> DQQLVDQLSQLKLNVKMLDNRAGENGVDCAALGADWASCNRVLFTLSNDGQAIDGKDWVIYFHSPRQTLRVDNDQFKIAHLTGDLYKLEPTAKFSGFPAGKAVEIPVVAEYWQLFRNDFLPRWYATSGDAKPKMLANTDTENLDQFVAPFTGDQWKRTKDDKNILMTPASRFVSNADLQTLPAGALRGKIVPTPMQVKVHAQDADLRKGVALDLSTLVKPAADVVSQRFALLGVPVQTNGYPIKTDIQPGKFKGAMAVSGAYELKIGKKEAQVIGFDQAGVFYGLQSILSLVPSDGSGKIATLDASDAPRFPYRGIFLDVARNFHKKDAVLRLLDQMAAYKLNKFHFHLSDDEGWRIEIPGLPELTEVGGQRCHDLSETTCLLPQYGQGPDVYGGFFSRQDYIDIIKYAQARQIEVIPEIDMPAHARAAVVSMEARYKKLHAAGKEQEANEFRLVDQTDTSNTTSVQFFNRQSYLNPCLDSSQRFVDKVIG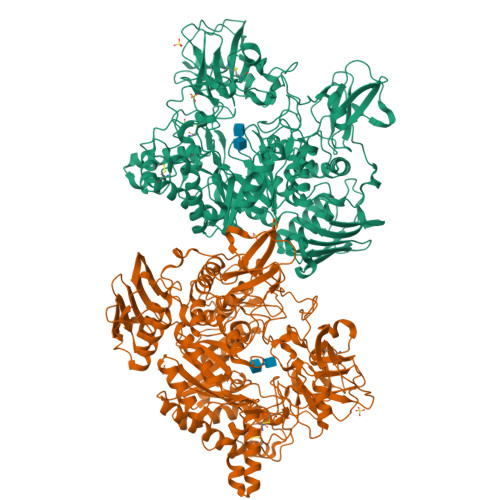EIAQMHKEAGQPIKTWHFGGAEAKNIRLGAGYTDKAKPEPGKGIIDQSNEDKPWAKSQVCQTMIKEGKVADMEHLPSYFGQEVSKLVKAHGIDRMQAWQDGLKDAESSKAFATSRVGVNFWDTLYWGGFDSVNDWANKGYEVVVSNPDYVYMDFPYEVNPDERGYYWGTRFSDERKVFSFAPDNMPQNAETSVDRDGNHFNAKSDKPWPGAYGLSAQLWSETQRTDPQMEYMIFPRALSVAERSWHRAGWEQDYRAGREYKGGETHFVDTQALEKDWLRFANILGQRELAKLDKGGVAYRLPVPGARVAGGKLEANIALPGLGIEYSTDGGKQWQRYDAKAKPAVSGEVQVRSVSPDGKRYSRAEKV> DAIIQMIVELLK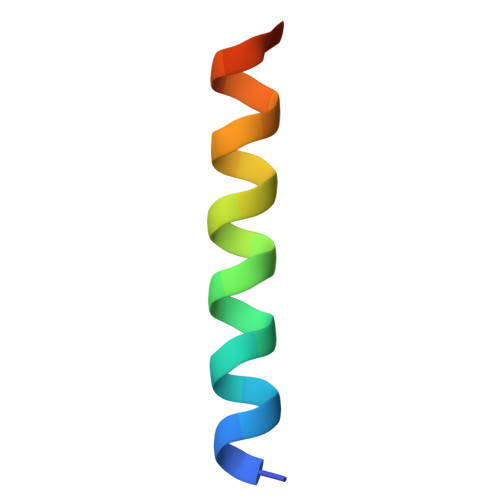RVGDQWEEEQSLAS> VVGGEDAKPGQFPWQVVLNGKVDAFCGGSI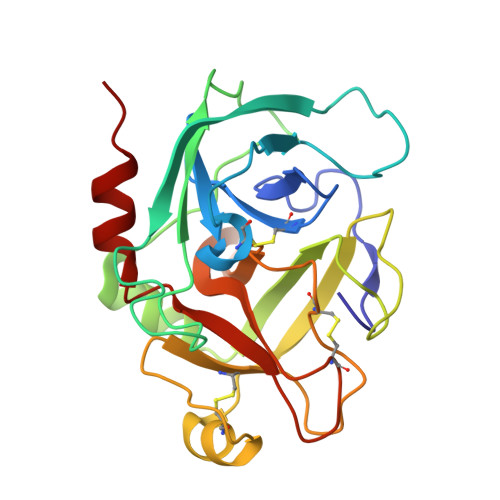VNEKWIVTAAHCVETGVKITVVAGEHNIEETEHTEQKRNVIRIIPHHNYNAAINTYNHDIALLELDEPLVLNSYVTPICIADKEYTNIFLKFGSGYVSGWGRVFHKGRSALVLQYLRVPLVDRATCLRSTKFTITNNMFCAGFHEGGRDSCQGDSGGPHVTEVEGTSFLTGIISWGEECAMKGKYGIYTKVSRYVNWIKEKTKLT2-(2-METHYLPHENYL)-1H-INDOLE-5-CARBOXIMIDAMIDE | C16 H15 N3 | 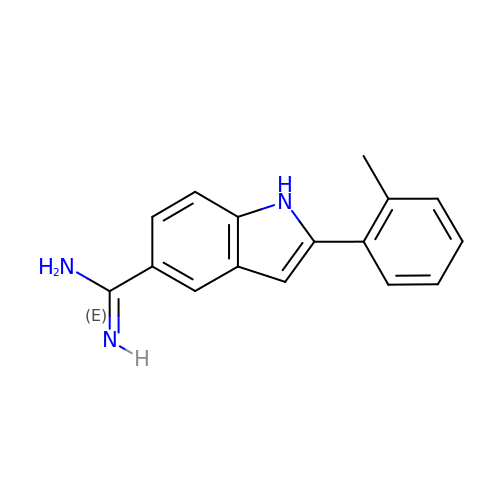YOZKTHGEOJHIDP-UHFFFAOYSA-N>[4x]MAHHHHHHHRSEQIAAVRRMVEAYNTG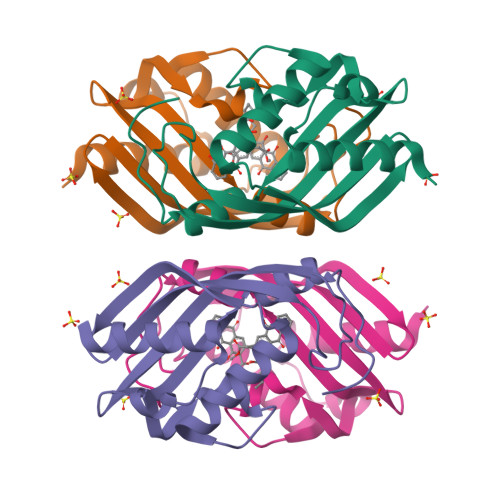KTDDVADYIHPEYMNPGTLEFTSLRGPELFAINVAWVKKTFSEEARLEEVGIEERADWVRARLVLYGRHVGEMVGMAPTGRLFSGEQIHLLHFVDGKIHHHRDWPDYQGTYRQLGEPWPETEHRRP>MRALVSKARL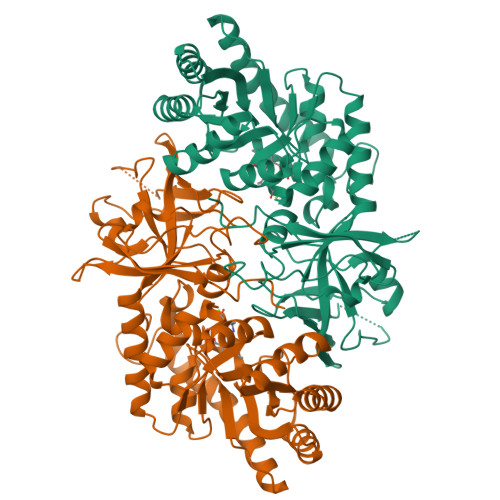AHSVGGRASQATRCAATISASRAPAHLGDALHDVDTPALILDLDAFDRNCEKLKGVMAGFPGVAVRPHAKAHKCAEVARRQLQLLGAKGVCCQKVIEAEAMAEGGVSDLLLSNEVIAPRKIDRLVGLAAAGARVGVCYEREDNLRQLNAAAAARGTHLDVLVELNVGQDRCGVNSADEVVQLARAAAGLDNVRFAGIQAYHGGLQHVRDPRDRAQRVGQVVGRARAAVDALKAAGLPCDTVTGGGTGTYRVEAASGVFTEVQPGSFAFSDADYARNLQEDGGVGEWEQSLWVLTQVMSVTPARGLAVVDAGTKAVSLDSGPPRLPPAFEAAYGTMMEYGSGGDEHGKLMWPQGAYQLPMSLPEVGSLLLLQPGHCDPTVNLYDWLVAARRQQGGQQQGGVDGWRVEAVWPIRGRGPGQ[4x]>MELYRDPSQPIEVRVRDLLSRMTLEEKVAQLGSVWGYELIDERGKFSREKAKELLKNGIGQITRPGGSTNLEPQEAAELVNEIQRFLVEETRLGIPAMIHEECLTGYMGLGGTNFPQAIAMASTWDPDLIEKMTTAVREDMRKIGAHQGLAPVLDVARDPRWGRTEETFGESPYLVARMGVSYVKGLQGEDIKKGVVATVKHFAGYSASEGGKNWAPTNIPEREFKEVFLFPFEAAVKEANVLSVMNSYSEIDGVPCAANRKLLTDILRKDWGFEGIVVSNYFAVKVLEDYHRIARDKSEAARLALEAGIDVELPKTECYQYLKDLVEKGIISEALIDEAVTRVLRLKFMLGLFENPYVEVEKAKIESHRDIALEIARKSIILLKNDGILPLQKNKKVALIGPNAGEVRNLLGDYMYLAHIRALLDNIDDVFGNPQIPRENYERLKKSIEEHMKSIPSVLDAFKEEGIEFEYAKGCEVTGEDRSGFEEAIEIAKKSDVAIVVVGDKSGLTLDCTTGQSRDMANLKLP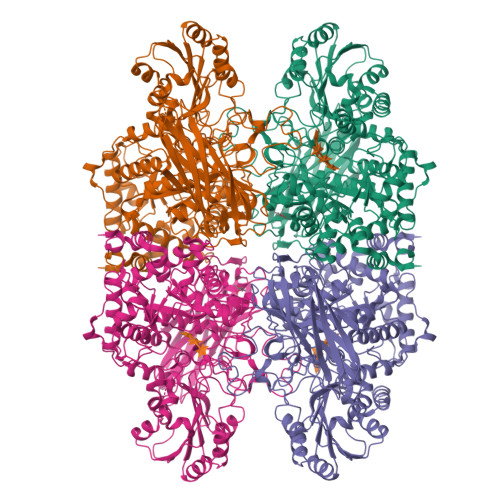GVQEELVLEVAKTGKPVVLVLITGRPYSLKNVVDKVNAILQVWLPGEAGGRAIVDIIYGKVNPSGKLPISFPRSAGQIPVFHYVKPSGGRSHWHGDYVDESTKPLFPFGHGLSYTKFEYSNLRIEPKEVPPAGEVVIKVDVENIGDRDGDEVVQLYIGREFASVTRPVKELKGFKRVSLKAKEKKTVVFRLHMDVLAYYNRDMKLVVEPGEFKVMVGSSSEDIRLTGSFSVVGEKREVVGMRKFFTEACEEAA[2x]> MSWWWAGAIGAAKKRSDEDEALPKHSSVALIVGVTGIVGNSLAEILPLADTPSGPWKVYGVARRPRPAWNEDNPINYIRCDISDPKDTQEKLSPLTDITHVFYVTWANRSTEVERCEANGKMLKNVLDVVIPNCPDLKHISLQTGRKHYVGPFELIGKIETHDPPFTEDLPRLKFDNFYYTQEDLLFEEVEKKEGLTWSVHRPGNIFGFSPYSMMNLVGTLCVYAAICKH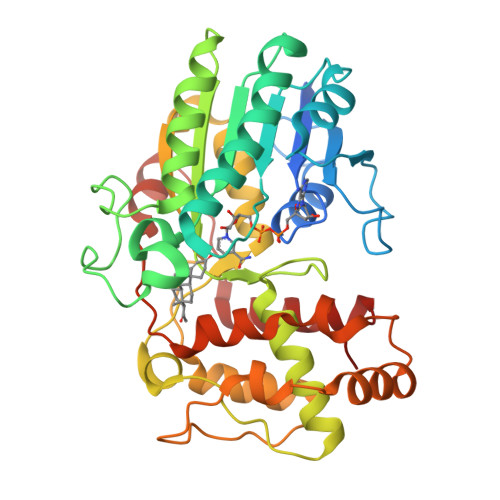EGKVLRFPGCKAAWDGYSDCSDADLIAEHHIWAAVDPYAKNEAFNVSNGDVFKWKHFWKVLAEQFGVECGEYEEGENLKLQDLMKGKEPVWEEIVRENGLASTNLEDVAVWWFSDAVLDIPCPLDSMNKSKEHGFLGFRNSKNSFISWIDKAKAYKIVP> MTTAKKRKLPSDLHDVEVGIKRPRISGQEITLLNSNPYPDNFYVGQAIGNGSCFFDSFRQSLEQQTGEQVTAEKLRNDCREFAQKNPPKWFTNAIVNSHD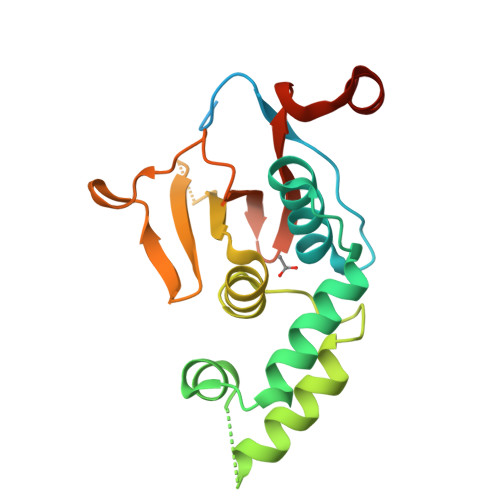NNGQHRSETVDNYTADIMRNSRWGDPDVEGRILCEKYKVKLHVIENQTVDNQDLSLHELIDNSGSKSAGEYNKVDYDDSSTVHIINKGGLHFEPLLDRNKSSAKQLQEQEDFLLA(1R,2S,4S,5R)-2-(2,3,4,5,6-pentafluorophenyl)methyl-1,4,5-trihydroxy-3-oxocyclohexane-1-carboxylic 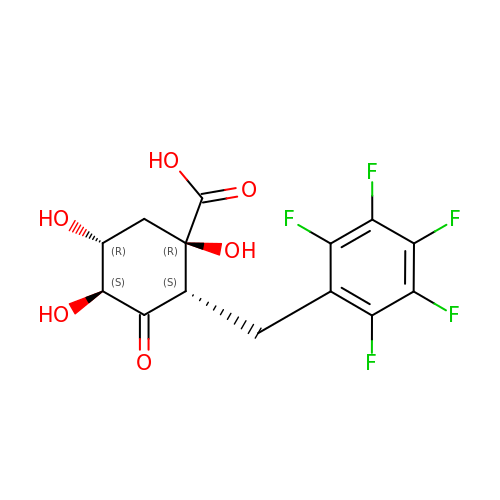acid | C14 H11 F5 O6 | ZNZHQTVBMHBUCF-GLOYCNQYSA-N>[6x]MFEEINDFETAFKRLLNEVLEFDLQNPLKDVKKVLCIEPHPDDCVIGMGGTIKRLTDRGIEVIYICMTDGYMGTTDENITGHELAQIRRKEEEESAKMLGVKKIYWLNYRDTELPYSREVRKDLVKIIRKEKPDGVFLPDPWLPYEAHPDHRATGFLALDAVAFSPLP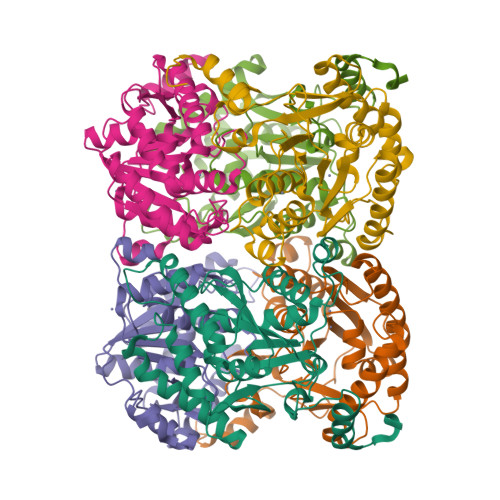NFSNIDLDIGLKPHSVSFIGLYYTSRPNYFVDITDVMDLKLKAIRAHKSQFPDDIWETWEPFLRTVALYYGQKAGVKYAEGFRIMPGLFYHITPFAELI> MGHHHHHHGNHEKMKAVPVLHGEGNRLFKLGRYEEASSKYQEAIICLRNLQTKEKPWEVQWLKLEKMINTLILNYCQCLLKKEEYYEVLEHTSDILRHHPGIVKAYYVRARAHAEVWNEAE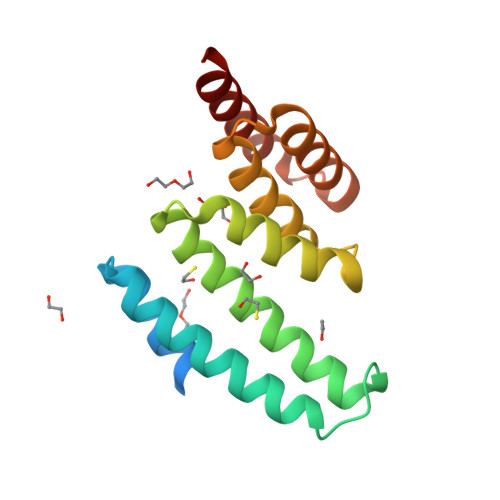AKADLQKVLELEPSMQKAVRRELRLLENRMAEKQ> GAMGQTSTRWTPTTEQIKILKELYYNNAIRSPTADQIQKITARLRQFGKIEGKNVFYWFQNHKARERQKKRFNG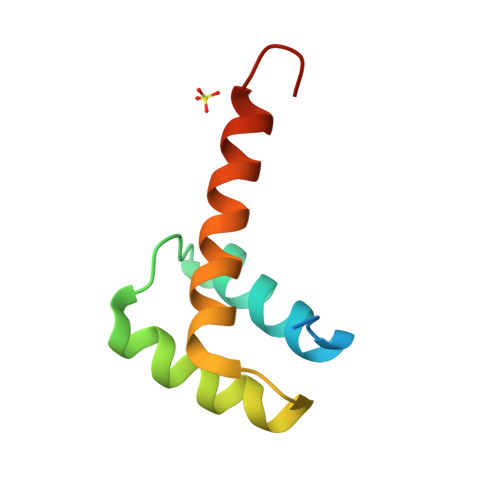GS>GAQMDAESIEWKLTANLRNGPTFFQPLADSIEPLQFKLIGSDTVATAFPVFDTKYIPDSLINYLFKLFNLEIESGKTYPQLHSLTKQGFMNYWFHSFAVVVLQTDEKFIQDNQDWNSVLLGTFYIKPNYAPRCSHNCNAGFLVNGAHRGQKVGYRLAQVYLNWAPLLGYKYS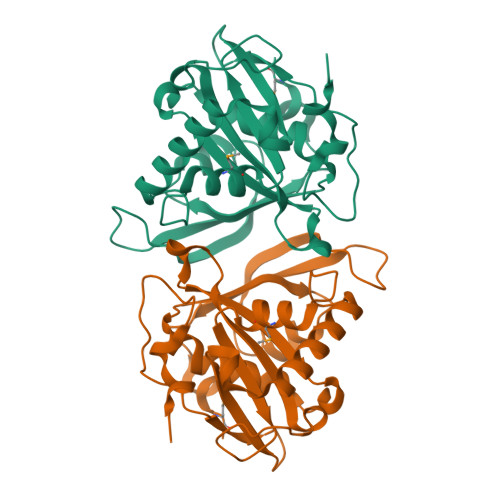IFNLVFVTNQASWKIWDKLNFQRIGLVPHAGILNGFSEPVDAIIYGKDLTKIEPEFLSME[3x]> MTQPASSRVVFDPSNPTTFSVEAIAAYTPVALIRLLNASGPLQPGHRVDIADARSIYTVGAAASAARARANHNANTIRRTAMFAETDPMTWLRPTVGLKRTFNPRIIRPQPPNPSMSLGISGPTI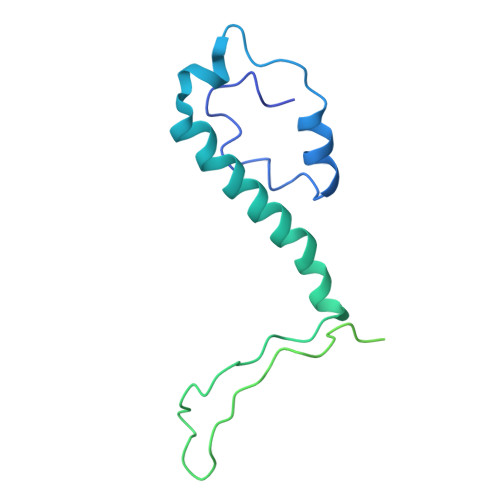LPQKTQSADQSALQQPAALAFSGSSPQHPPPQTTSASVGQQQHVVSGSSGQQPQQGAQSSTVQPTTGSPPAAQGVPQSTPPPTQNTPQGGKGQTLSHTGQSGNASRSRRV4-methoxybenzamide | C8 H9 N O2 | 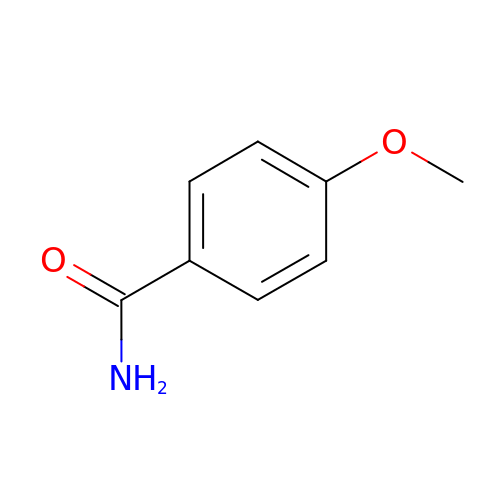GUCPYIYFQVTFSI-UHFFFAOYSA-N>[2x]MGHSSSVTGVAFSPDGQTIASASDDKTVKLWNRNGQLLQTLTGHSSSVTGVAFSPDGQTIASASDDKTVKL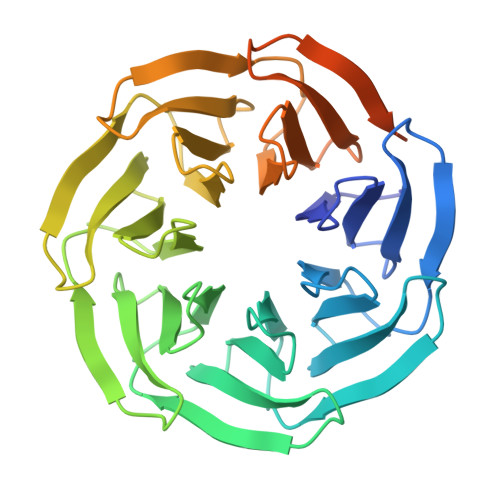WNRNGQLLQTLTGHSSSVTGVAFSPDGQTIASASDDKTVKLWNRNGQLLQTLTGHSSSVTGVAFSPDGQTIASASDDKTVKLWNRNGQLLQTLTGHSSSVTGVAFSPDGQTIASASDDKTVKLWNRNGQLLQTLTGHSSSVTGVAFSPDGQTIASASDDKTVKLWNRNGQLLQTLTGHSSSVTGVAFSPDGQTIASASDDKTVKLWNRNGQLLQTLTGHSSSVTGVAFSPDGQTIASASDDKTVKLWNRNGQLLQTLT>[2x]GPGSEFQRPTMESVRNFEQWQSQRNQLQGAMQQFNQRYLYSASMLAAENDPYGPLPPGWEKRVDSTDRVYFVNHNTKTTQWEDPRTQGLQNEEPLPEGWEIRYTREGVRYFVDHNTRTTTFKDPRNGKSSVTKGGPQIAYERGFRWKLAHFRYLCQSNALPSHVKI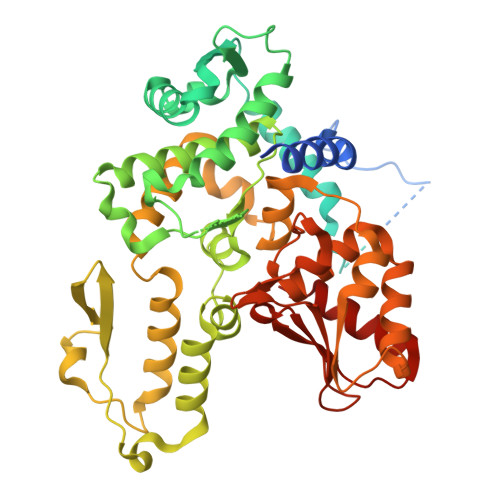NVSRQTLFEDSFQQIMALKPYDLRRRLYVIFRGEEGLDYGGLAREWFFLLSHEVLNPMYCLFEYAGKNNYCLQINPASTINPDHLSYFCFIGRFIAMALFHGKFIDTGFSLPFYKRMLSKKLTIKDLESIDTEFYNSLIWIRDNNIEECGLEMYFSVDMEILGKVTSHDLKLGGSNILVTEENKDEYIGLMTEWRFSRGVQEQTKAFLDGFNEVVPLQWLQYFDEKELEVMLCGMQEVDLADWQRNTVYRHYTRNSKQIIWFWQFVKETDNEVRMRLLQFVTGTCRLPLGGFAELMGSNGPQKFCIEKVGKDTWLPRSHTCFNRLDLPPYKSYEQLKEKLLFAIEETEGFGQE>[4x]SLSPSARRVQGALETRGFGHLKVVELPASTRTAKEAAQAVGAEVGQIVKSLVYGGEKGAYLFLVSGKN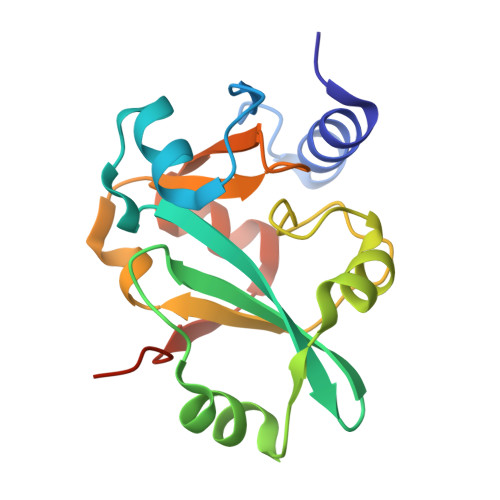RLDLGKATRLVGGPLLEADKWAVAALTGFDAGGVPPVGHNTPLPAYLDEDLLGYPEVWAAGGTPRALFRATPKELLALTGAQVADLKEGLEHHHHHH>[8x]KRAHHNA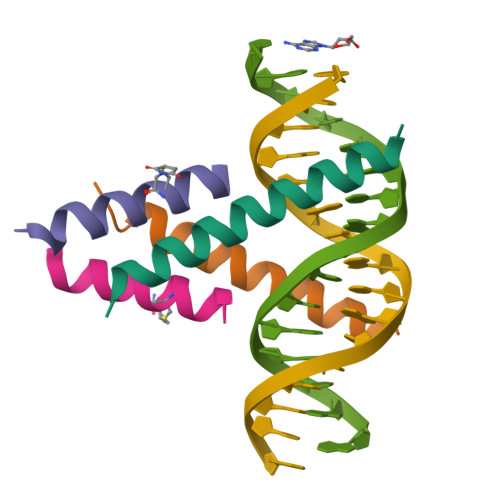LERKRRDHIKDSFHKLRDSVP;>[8x]XSRAQILCKATEYIQYMRRKN> MLPPDILQNGEFETIYFQTNPTYIKSPIHIPKSTIGKPDTVKIRHFFALLHQDLVVLGLEVFVYLQIYSDFVEKYVYVSKCDTVGLEKSTIKIGKVIGPVLQYIINYNGYKIKMKNLDEKSKDLSDPSTLVR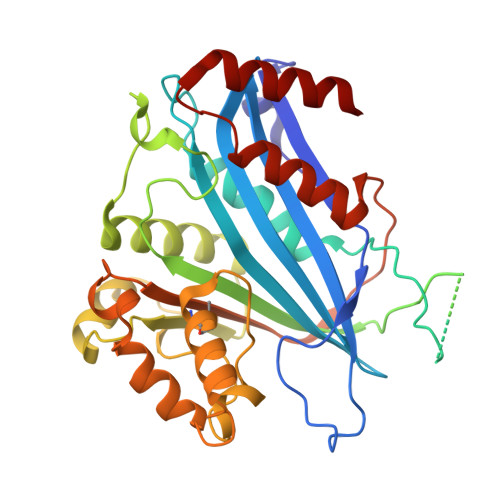LQRLRDKLPDIYPNLPYYNDIPPKEECIEYRTLPKTQNLRLCVFTKPAKEYLFPNSAKNPYKALLNGQSLLRWWISIIDSITKGWNNHKLMIPGADKYATRKFIEKYSDWSEGHIFKKDGLAVQAIPLFPDDPKGRFLELVIVECRYGKMTVSRFYQELAYRQEFLLGDCVSLIGCCKENLEVTYHDDLVSTVTISEYKEFMNLLKLVDFSDRVEVSNFVSNYRKSK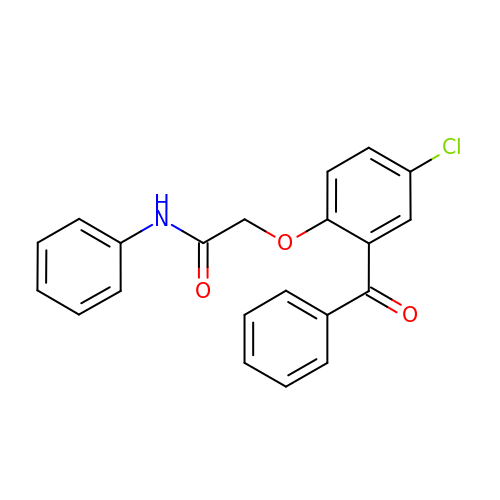2-[4-chloro-2-(phenylcarbonyl)phenoxy]-N-phenylacetamide | C21 H16 Cl N O3 | DTGVSZSMDOMAEB-UHFFFAOYSA-N>YPITGDGVNCRSGPGTSYSVVKSYQKGADVAITCQAPGTDVKGDNIWDKTADGCYVADYYIKTGSSSYVTAKCD[2x]

Muramidases are N-acetylmuramide glycanhydrolases which cleave the β-1,4-glycosidic bond between N-acetylmuramic acid (NAM) and N-acetylglucosamine (NAG) in the carbohydrate backbone of the bacterial cell-wall peptidoglycan. Here, the identification, characterization and X-ray structure of a novel fungal GH24 muramidase from Trichophaea saccata is first described, in which an SH3-like cell-wall-binding domain (CWBD) was identified by structure comparison in addition to its catalytic domain. A ‘domain-walking’ approach, searching for other sequences with a domain of unknown function appended to the CWBD, was then used to identify a group of fungal muramidases that also contain homologous SH3-like cell-wall-binding modules, the catalytic domains of which define a new GH family. The properties of some representative members of this family are described as well as X-ray structures of the independent catalytic and SH3-like domains of the Kionochaeta sp., Thermothielavioides terrestris and Penicillium virgatum enzymes.

Attempts were made to crystallize the full-length enzymes from T. terrestris and P. virgatum. The crystals of the T. terrestris enzyme contained only the catalytic GH184 domain, which was closely similar to that from Kionochaeta sp. The P. virgatum crystal, in contrast, only contained the SH3-like CWBD, which was similar in fold to the GH24 CWBD. Again, the aim was to crystallize the full-length enzyme, but as for the T. terrestris protein the domains were cleaved during the crystallization process. In contrast to T. terrestris, for this protein the crystals contained only the N-terminal CWBD. Its structure is similar to the CWBD from the T. saccata GH24 muramidase. There are two independent monomers in the asymmetric unit with a zinc ion bound between them; this zinc ion is a crystallization artefact. Two disulfide bridges are present in the same location as in TsCWBD, which could add to the domain stability; however, they are not likely to be essential because the structurally similar SH3 domains lack these disulfide bridges. The second disulfide bridge could, however, play a role in target specificity because it brings the C-terminal loop into close proximity to the binding pocket. In addition, two ethylene glycol molecules are bound to each monomer.>[2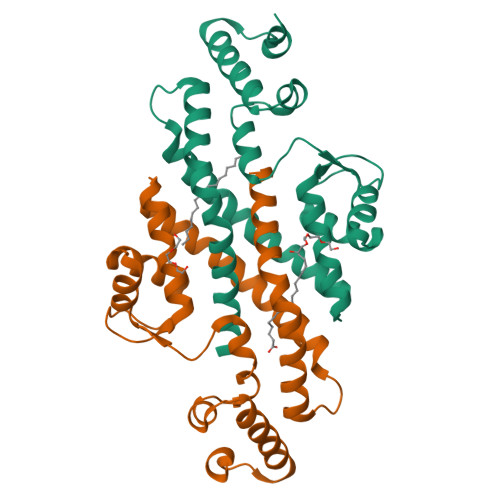x]MRGSHHHHHHGSMTDHVREADDANIDDLLGDLGGTARAERAKLVEWLLEQGITPDEIRATNPPLLLATRHLVGDDGTYVSAREISENYGVDLELLQRVQRAVGLARVDDPDAVVHMRADGEAAARAQRFVELGLNPDQVVLVVRVLAEGLSHAAEAMRYTALEAIMRPGATELDIAKGSQALVSQIVPLLGPMIQDMLFMQLRHMMETEAVNAGERAAGSSP In this report, we show the hypothetical protein CT622, which had previously been detected in the host cell cytosol is a T3S effector and we identify a novel putative chaperone protein for this effector. Our results converge to identify CT622 as a secreted protein that plays multiple and crucial roles in the initiation and support of the C. trachomatis growth cycle. In order to gain more insights into the molecular mechanism of CT622 function during Chlamydia infection, we undertook a structural analysis of CTL0886, the CT622 ortholog in the strain C. trachomatis L2 434/Bu. CT622 is the first chlamydial effector identified to date whose genetic disruption has such a strong impact on bacterial development in cell culture, without being fully lethal.

Indeed, LC-MS/MS analysis (data not shown) of the excised bands suggested that two unique CTL0886FL domains were present spanning residues 94–334 (CTL0886N) and residues 353–651 (CTL0886C). While equally poor diffraction was initially obtained with CTL0886C crystals, reductive methylation of surface exposed lysines enabled the growth of cubic crystals that diffracted synchrotron X-rays to 1.90 Å resolution. The structure of CTL0886C was determined using selenomethionine-labeled recombinant protein (also dimethylated) by Se-SAD and refined against the native high-resolution dataset. The final model is comprised of a single polypeptide in the asymmetric unit, 1 sulfate anion and 98 water molecules. The CTL0886C structure is comprised of 13 α-helices spanning two separate domains. Domain 1 consists of helices α1–7 arranged in a 7 helix bundle (residues 353–517). Helices α8–13 of domain 2 adopt an intertwined, globular fold with the later 3 helices (α11–13) wrapping around helices α8–10. Upon inspection of the 2Fo-Fc electron density map, four lysine residues (446, 463, 490, and 579) were modeled as dimethyl-lysine. For domain 1, each of these structures (as well as the next 10 scoring hits) are all members of the polyprenyl transferase (PTS) family. CTL0886C domain 1 is, however, lacking several α-helices typically found within the PTS family, including those involved in dimerization and extended regions typically found within the active site of PTS family enzymes (e.g., Asp-rich motifs).

> SLLLDDVDNEMAAIAMQGFRSMIEQFNVNNPATAKELQAMEAQLTAMSDQLVGADGELPAEIQAIKDALAQALKQPSADGLATAMGQVAFAAAKVGGGSAGTAGTVQMNVKQLYKTAFSSTSSSSYAAALSDGYSAYKTLNSLYSESRSGVQSAISQTANPALSRSVSRSGIESQGRSADASQRAAETIVRDSQTLGDVYSRLQVLDSLMSTIVSNPQANQEEIMQKLTASISKAPQFGYPAVQNSVDSLQKFAAQLEREFVDGERSLAESQENAFRKQPAFIQQVLVNIASLFSGYLS>[4x]STDISTVASPLFEGTEGCFLLYDASTNAEIAQFNKAKCATQMAPDSTFDIALSLMAFDAEIIDQKTIFKWDKTPKGMEIWNSNHTPKTWMQFSVVWVSQEITQKIGLNKIKNYLKDFDYGNQDFSGDKERNNGLTEAWLESSLKISPEEQIQFLRKIINHNLPVKNSAIENTI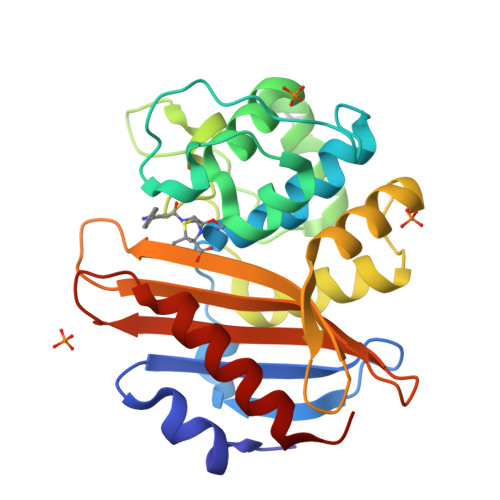ENMYLQDLDNSTKLYGKTGAGFTANRTLQNGWFEGFIISKSGHKYVFVSALTGNLGSNLTSSIKAKKNAITILNTLNL(5S)-2-{[(1S)-1-(2-fluorophenyl)ethyl]amino}-5-methyl-5-(trifluoromethyl)-1,3-thiazol-4(5H)-one 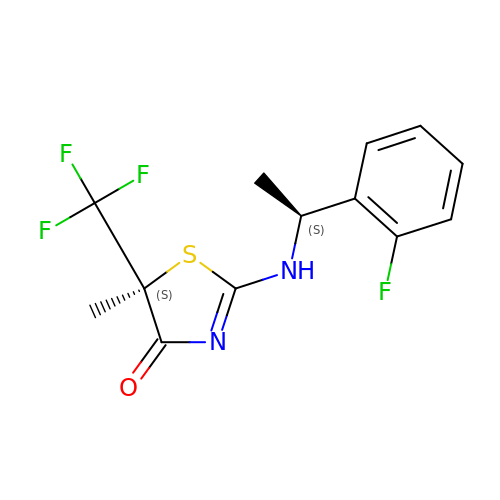| C13 H12 F4 N2 O S | KNHNFKZUNFPPQE-MADCSZMMSA-N> SH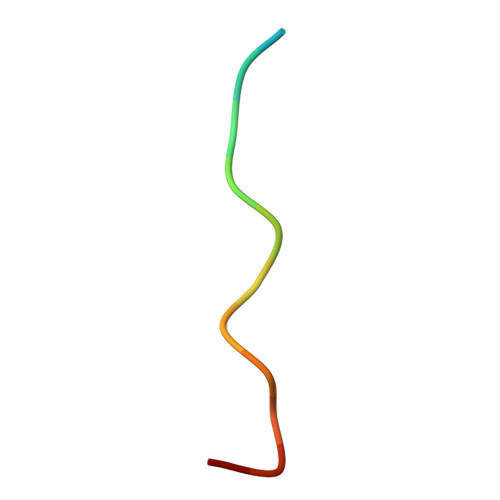KHDPLPYPHFLL7-bromanyl-3-[[4-oxidanyl-1-[(3~{R})-3-phenylbutanoyl]piperidin-4-yl]methyl]thieno[3,2-d]pyrimidin-4-one | C22 H24 Br N3 O3 S | 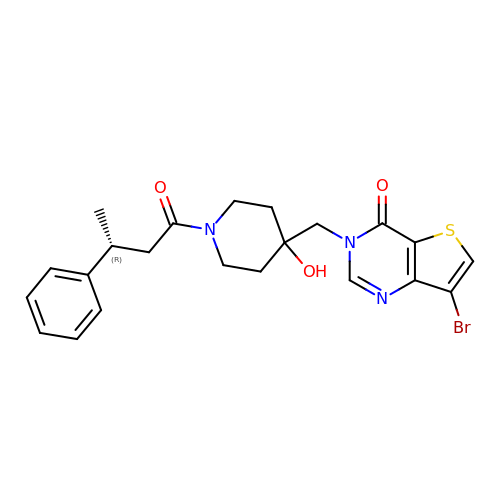NRRXSEFLOFZNSO-OAHLLOKOSA-N> MTPESVMMMGTEAMKVALALAAPLLLVALITGLIISILQAATQINEMTLSFIPKIVAVFIAI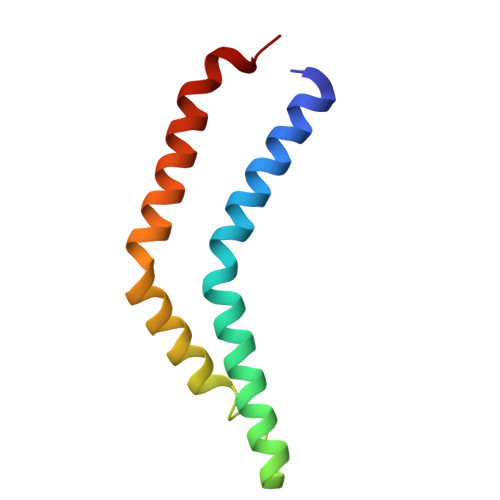IVAGPWMLNLLLDYVRTLFSNLPYIIG> GSHMNDHINLKVAGQDGSVVQFKIKRHTPLSKLMKAYCERQGLSMRQIRFRFDGQPINETDTPAQLEMEDEDTIDVFQQQTGGVPESSL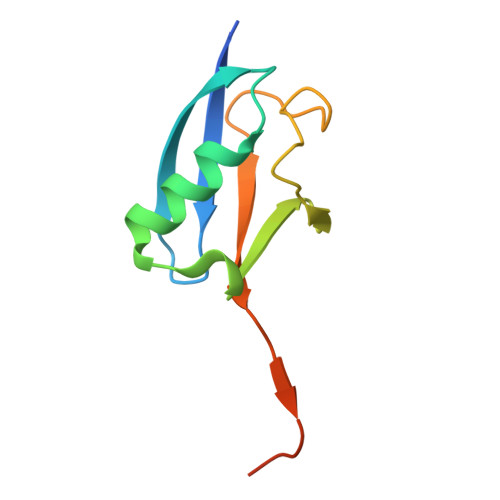AGHSF> MNQIWLKVCAASDMQPGTIRRVNRVGAAPLAVYRVGDQFYATEDTCTHGIASLSEGTLDGDVIECPFHGGAFNVCTGMPASSPCTVPLGVFEVEV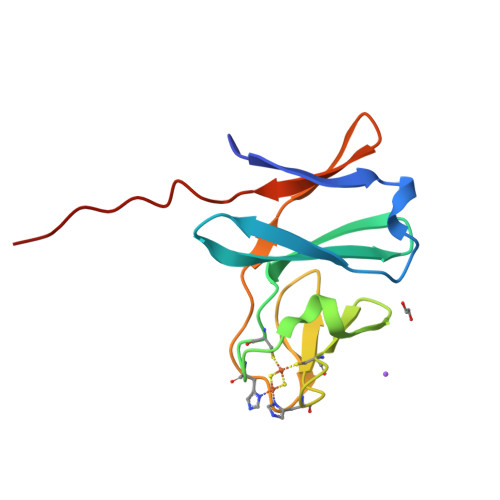KEGEVYVAGEKKLEHHHHHH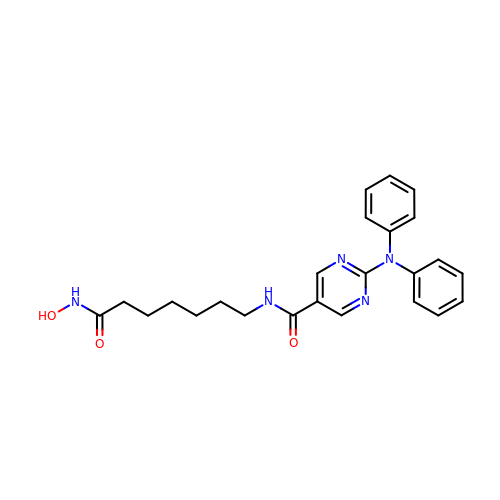2-(diphenylamino)-N-[7-(hydroxyamino)-7-oxoheptyl]pyrimidine-5-carboxamide | C24 H27 N5 O3 | QGZYDVAGYRLSKP-UHFFFAOYSA-N> MHHHHHHSSGRENLYFQGPFDAIKQPNRSEEEVTQLAEDFKDWSKASNGWRYSFITANEKEAVEDFSISGYQTANDYLRATDTSTWGVAGADARQYIRTVKSALNKLPKYKGTAYRGTWVKLSLLNKLEEGDVLVEPAFTSTSTLPEVAKRFSVVHPNSPQRLKRVLFEVKINQGGHTIAGLSEYSKEAEVLFAPNAHFRITQIERTS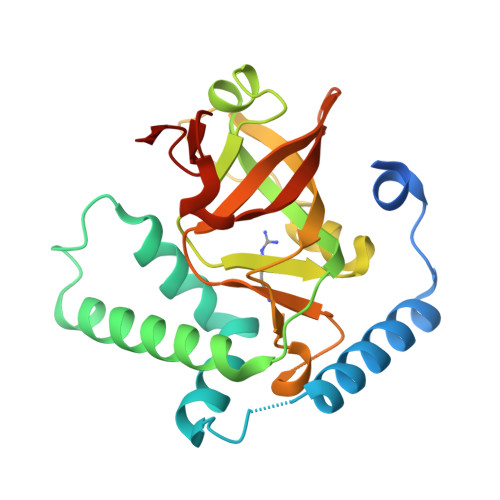NHTYIGVETVKASAVKNTQKYNLYSGEEVEA>MGKVNVAKLRYMSRDDFRVLTAVEMGMKNHEIVPGSLIASIASLKHGGCNKVLRELVKHK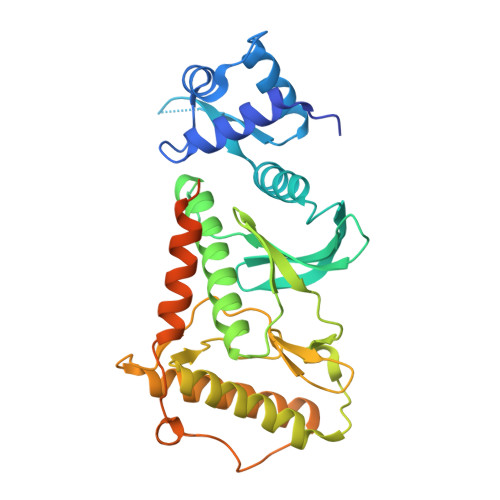LIAWERTKTVQGYRLTNAGYDYLALKTLSSRQVVESVGNQMGVGKESDIYIVANEEGQQFALKLHRLGRTSFRNLKNKRDYHKHRHNVSWLYLSRLSAMKEFAYMKALYERKFPVPKPIDYNRHAVVMELINGYPLCQIHHVEDPASVYDEAMELIVKLANHGLIHGDFNEFNLILDESDHITMIDFPQMVSTSHPNAEWYFDRDVKCIKDFFMKRFSYESELFPTFKDIRREDTLDVEVSASGYTKEMQADDELLHPLGPDDKNIETKEGSEFSFSDGEVAEKAEVYGSENE[2x]> GHMMRKLGLIAGGGALPVELASHCEAAGRAFAVMRLRSFADPSLDRYPGADVGIGEFGKIFKALRAEGCDVVCFAGNVS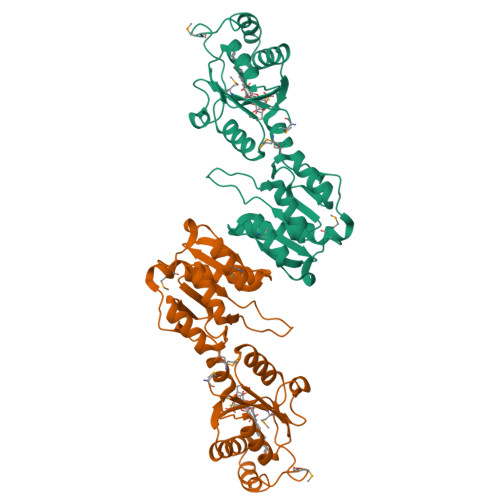RPDFSALMPDARGLKVLPSLIVAARKGDDALLRRVLDEFEKEGFEIEGAHEVMGEMTLPRGRLGKVSPAPEHMADIDKALDVAREIGRLDIGQGAVVCEGLVLAVEAQEGTDAMLRRVADLPEAIRGRAERRLGVLAKAPKPIQETRVDLPTIGVATIHRAARAGLAGIVGEAGRLLVVDREAVIAAADDLGLFVLGVDPQERP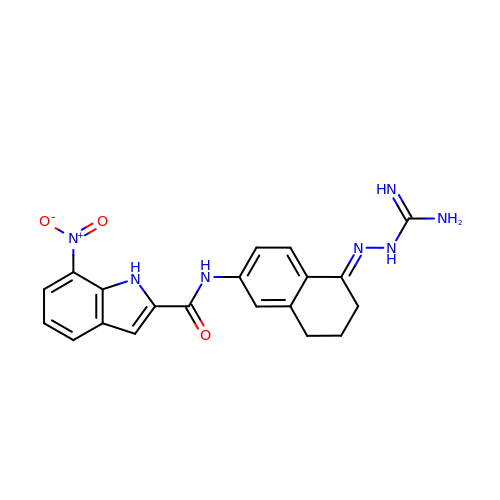(E)-N-(5-(2-CARBAMIMIDOYLHYDRAZONO)-5,6,7,8-TETRAHYDRONAPHTHALEN-2-YL)-7-NITRO-1H-INDOLE-2-CARBOXAMIDE | C20 H19 N7 O3 | CFOWEKJDEFRRLQ-MFKUBSTISA-N>[2x]PTPVEVSQLTYNADTIGNWVPPTELKQTYTQDITGLKPN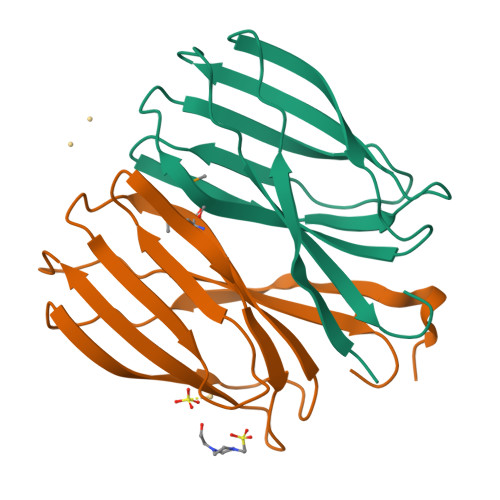SKFIIVPYMDRVSSEVLQKCTITCNEVDAVGSISYFDTSAIKCDGYISFQANSIGEATFTLVTDYQGAVDPKPYQYRIIRAIVGNN>[2x]MDGFSRRRMLMTGGALGAVGALGAATRALARPLWTWSPSASVAGTGVGVDPEYVWDEEADPVLAAVIDRGEVPAVNALLKQWTRNDQALPGGLPGDLREFMEHARRMPSWADKAALDRGAQFSKTKGIYVGALYGLGSGLMSTAIPRESRAVYYSKGGADMKDRIAKTARLGYDIGDLDAYLPHGSMIVTAVKTRMVHAAVRHLLPQSPAWSQTSGGQKIPISQADIMVTWHSLATFVMRKMKQWGVRVNTADAEAYLHVWQVSAHMLGVSDEYIPATWDAANAQSKQVLDPILAHTPEGEALTEVLLGIVAELDAGLTRPLIGAFSRYTLGGEVGDMIGLAKQPVLERLIATAWPLLVAFREGLIPLPAVPAVLWTLEEALRKFVLLFLSEGRRIAIDIPDVNRPS

The second type of rubber oxygenase has been named latex clearing protein (Lcp). Controversial reports were published on the cofactor of Lcp from Streptomyces sp. K30 (LcpK30) and G. polyisoprenivorans VH2 (LcpVH2)23, 24 but recently iron was detected in an almost 1:1 stoichiometry in pure preparations of LcpK30 and of LcpRr, and both Lcps were identified as b-type cytochromes. The typical, α-helical tertiary structure identifies LcpK30 as a member of the globin family. However, LcpK30 contains additional subdomains at the N- and C-termini beyond the globin core that form two caps located on opposite sides of the protein.

While screening for appropriate crystallisation conditions, diffracting crystals of LcpK30 were also obtained in an imidazole-containing buffer, and a structure of LcpK30 in these crystals was determined to 1.48 Å resolution. These crystals belonged to the same space group (P1), albeit with slightly altered unit cell axes, again with two subunits per asymmetric unit. Most features of LcpK30 remained unchanged in this structure, including the positioning of the proximal axial ligand, His198, towards the haem moiety. However, remarkable differences were found for the distal haem ligand Lys167 and for Thr168. Both residues were shifted significantly, releasing the coordinative bond to the metal ion and breaking the secondary structure of helix E into two shorter helices connected by a loop. Concomitantly, the C-terminal helix Z5 was split into two parts connected by a short loop, helix Z6 rearranged towards the active site and the distal axial position at the haem iron was now occupied by an imidazole molecule from the crystallisation buffer. This structure showed an increased accessibility of the haem group, opening a direct access pathway to a cavity at the distal side of the haem group, and in spite of the presence of imidazole we suggest this to represent an open form of LcpK30. The observation of two similar conformations that differ in the nature of the distal haem ligands confirms a flexibility of the Lcp structure at the distal haem site and suggests that Lcp is a member of the hexa-coordinate haemoglobin subfamily that can switch between a hexa- and penta-coordinated form. The imidazole-bound Lcp could thus represent the structure of the otherwise penta-coordinated form that is able to bind dioxygen. The transition of LcpK30 to the open state generates a distinct, hydrophobic access channel that crosses the entire protein molecule leading past the active site haem group and exiting on the distal side. A single charged residue, Glu148, is located within this channel, at a distance of approximately 6 Å from the iron ion of the haem group.>MRRIYLNTYEQINKVKKILRKHLKNNLIGTYMFGSGVESGLKPNSDLDFLVVVSEPLTDQSKEILIQKIRPISKKIGDKSNLRYIELTIIIQQEMVPWNHPPKQEFIYGEWLQELYEQGYIPQKELNSDLTIMLYQAKRKNKRIYGNYDLEELLPDIPFSDVRRAIMDSSEELIDNYQDDETNSILTLCRMILTMDTGKIIPKDIAGNAVAESSPLEHRERILLAVRSYLGENIEWTNENVNL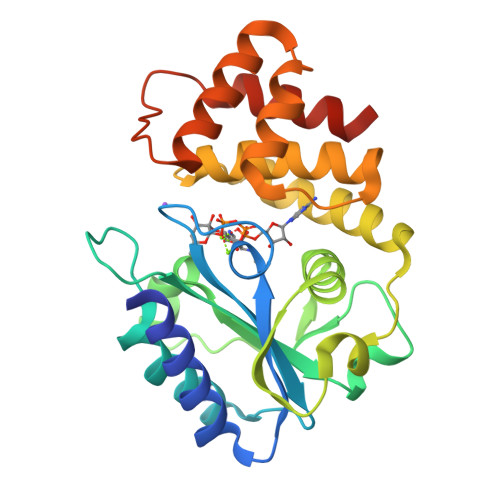TINYLNNRLKKLKGHHHHHH[2x]>QGAVRKATAAEIAALPRQKVELVDPPFVHAHSQVAEGGPKVVEFTMVIEEKKIVIDDAGTEVHAMAFNGTVPGPLMVVHQDDYLELTLINPETNTLMHNIDFHAATGALGGGGLTEINPGEKTILRFKATKPGVFVYHCAPPGMVPWHVVSGMNGAIMVLPREGLHDGKGKALTYDKIYYVGEQDFYVPRDENGKYKKYEAPGDAYEDTVKVMRTLTPTHVVFNGAVGALTGDKAMTAAVGEKVLIVHSQANRDTRPHLIGGHGDYVWATGKFNTPPDVDQETWFIPGGAAGAAFYTFQQPGIYAYVNHNLIEAFELGAAAHFKVTGEWNDDLMTSVL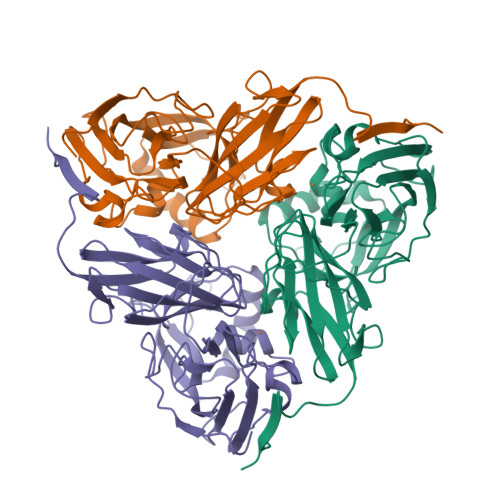APSGT[3x]>[6x]SNAMNALAATNRNFKLAARLLGLDSKLEKSLLIPFREIKVECTIPKDDGTLASFVGFRVQHDNARGPMKGGIRYHPEVDPDEVNALAQLMTWKTAVAKIPYGGAKGGIGCDPSKLSISELERLTRVFTQKIHDLIGIHTDVPAPDMGTGPQTMAWILDEYSKFHGYSPAVVTGKPIDLGGSLGRDAATGRGVMFGTEALLNEHGKTISGQRFVIQGFGNVGSWAAKLISEKGGKIVAVSDITGAIKNKDGIDIPALLKHTKEHRGVKGFDGADPIDPNSILVEDCDILVPAALGGVINRENANEIKAKFIIEAANHPTDPDADEILSKKGVVILPDIYANSGGVTVSYFEWVQNIQGFMWEEEKVNDELKTYMTRSFKDLKEMCKTHSCDLRMGAFTLGVNRVAQATILRGWGA

GDHs release the ammonium cation from glutamate in a reversible, NAD(P)+-dependent oxidative deamination reaction that yields 2OG. We have provided detailed structural and kinetic information about the functioning of AtGDH1, one of three mitochondrial NAD+-dependent GDHs in A. thaliana. The asymmetric unit of both crystal structures is comprised of a homohexameric oligomer with non-crystallographic 32 (D3) symmetry. A subunit of AtGDH1 is comprised of 411 amino acid residues (44.5 kDa) and can be subdivided into two domains.

In the AtGDH1-NAD+ complex, five subunits are in the open conformation (χ 70.2°–73.9°). The sixth subunit is in a closed conformation, characterized by the χ angle of 49.1°. The remarkably different conformation of AtGDH1 domain II in the open and closed states is correlated with other structural features. First, the closed conformation subunit contains 2OG, the GDH reaction product, bound in the active site (see below for details). Notably, 2OG had not been added to the protein preparation at any stage of purification or crystallization and, therefore, must have been captured from Escherichia coli cells during the recombinant protein expression. Each AtGDH1 subunit binds one molecule of the NAD+ coenzyme in a niche between domain I and domain II. In the closed subunit, the NAD cofactor is significantly more buried and, therefore, less exposed to the outer environment. The envelopment of NAD is primarily the result of the closing movement of domain II toward domain I, as the interactions of the coenzyme with domain II in the closed form are very similar to those in the open form. In our closed-conformation subunit (with 2OG in the active site), NAD+ is clearly oriented in a way that is compatible with hydride transfer to the Si face of nicotinamide. The distance between the C4 atom of NAD+ and C2 of 2OG is 4.2 Å in the closed structure.(2S)-2-[(3-hydroxy-5-oxo-4,5-dihydro-1,2,4-triazin-6-yl)sulfanyl]propanoic acid | C6 H7 N3 O4 S | 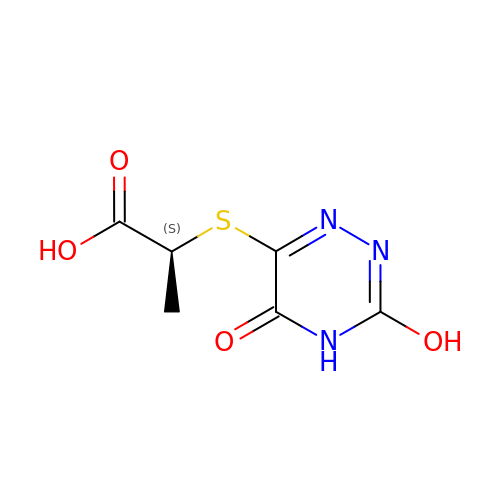RHHZZMNGKMZLIA-REOHCLBHSA-N>MWSHPQFEKTTNAGPLHPYWPQHLRLDNFVPNDRPTWHILAGLFSVTGVLVVTTWLLSGRAAVVPLGTWRRLSLCWFAVCGFIHLVIEGWFVLYYEDLLGDQAFLSQLWKEYAKGDSRYILGDNFTVCMETITACLWGPL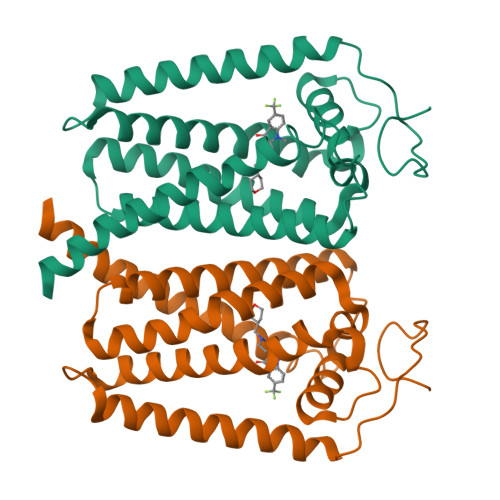SLWVVIAFLRQHPLRFILQLVVSVGQIYGDVLYFLTEHRDGFQHGELGHPLYFWFYFVFMNALWLVLPGVLVLDAVKHLTHAQSTLDAKATKAKSKKN[2x]>MQHTYPAQLMRFGTAARAEHMTIAAAIHALDADEADAIVMDIVPD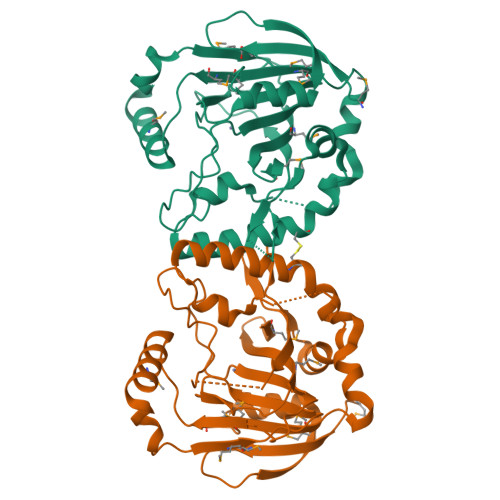GERDAWWDDEGFSSSPFTKNAHHAGIVATSVTLGQLQREQGDKLVSKAAEYFGIACRVNDGLRTTRFVRLFSDALDAKPLTIGHDYEVEFLLATRRVYEPFEAPFNFAPHCDDVSYGRDTVNWPLKRSFPRQLGGFLTIQGADNDAGMVMWDNRPESRAALDEMHAEYRETGAIAALERAAKIMLKPQPGQLTLFQSKNLHAIERCTSTRRTMGLFLIHTEDGWRMFD[2x]>MSASKEEIAALIVNYFSSIVEK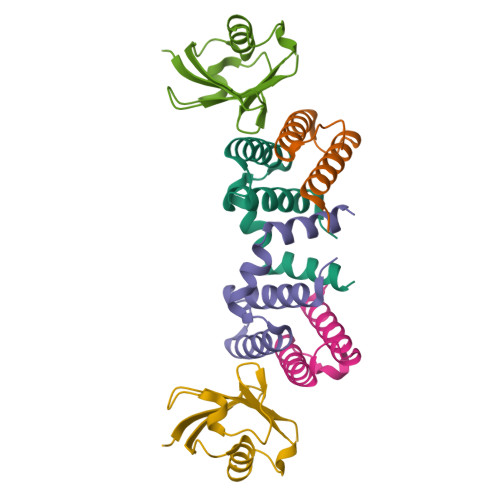KEISEDGADSLNVAMDCISEAFGFEREAVSGILGKSEFKGQHLADILNSA[4x];>[2x]NAAVHLTLKKIQAPKFSIEHDFSPSDTILQIKQHLISEEKASHISEIKLLLKGKVLHDNLFLSDLKVTPANSTITVMIKPN> GKRYIPFRTPRNPKSKHILA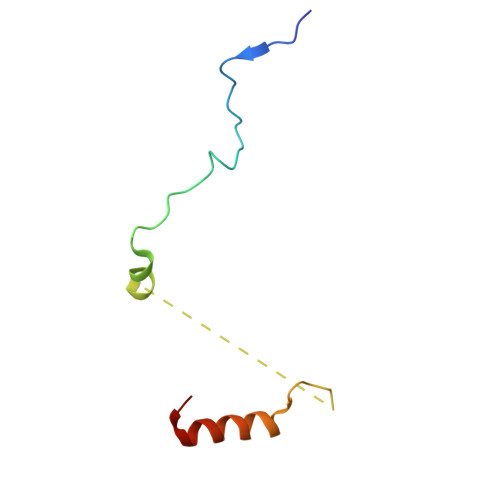TPPPLFAATALDARSFVWPPLHFVERRRRLLMEKNLL>[3x]GSENLYFQGSGSEELEKQALVYAVQVLLIALRAILQGDEKLFKLAEWAVELAIKALQNGDERQVQRAILFMQAVILIQI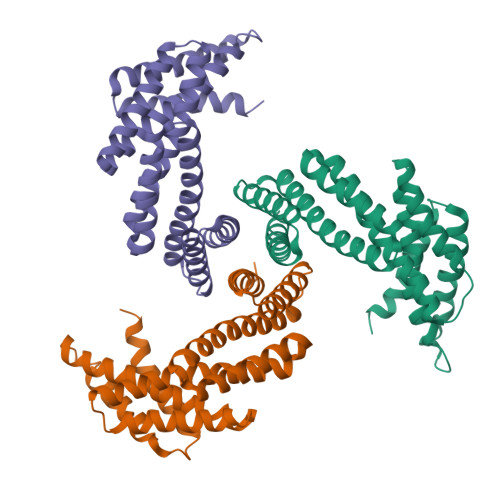VKEIAEEARKQGDEKLFELARWAIELAEKAIERGDEESVKRAILFMQAVILIQIVKKIAEKAKRQGDDKLFKLAEWAIELAERAIEEGDEEKVKRAILFMEAVILIQLVKEIAKKAKEQGDEELFQRAEEAIKDAEKAIEEGDEEKVKEAIKKMKEVIRIQERK>MGAFAPHFGSPFVRTSDYGKR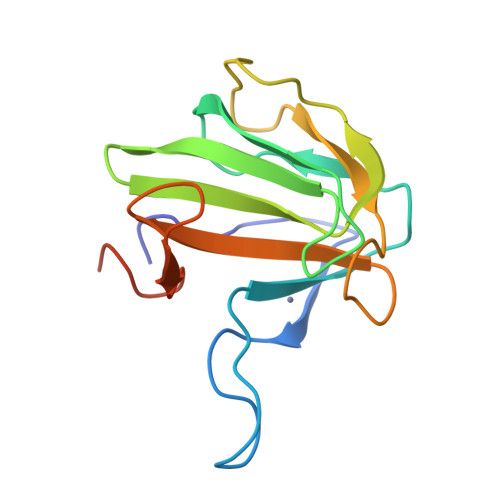PGLYGDFHTGIDYAAPTGTPIPAQYPGLVDWVQSSSIGLGEHVGIKVADNLWAMYGHMSRIRAKMGDKVKAGQIVGDVGSSGWSTGPAVHYELRKGGPNGQHVNPDTYGGAAGGSHHHHHH[5x]>MADPSSFASPEKFNIKHMHLKLHVDFTSRAIAASTSLTVRSLQDSLASLILDTKDLTIKKVAVNGKDATFALGTTHSFKGTPLEITLPFSLTRGQEVIVEIDSVTSPKSSALQWLNKEQTAGKIHPYLFSQCQATHCRSIIPCQDTPSVKFTYYSQVSVPKELMALMSALRDGELSEQSDSNRKIYRFKQNVPIPSYLIALVVGALEGRKVGPRTTIWTEKELLEPSVYEFAETEKMLKYAEDLAGPYVWGQYDLLILPPSFPYGGMENPCLTFVTPTVLAGDRSLASVIAHEISHSWTGNLVTNETWENFWLNEGHTVYLERRIDGRLYGEEFRQFKALGGWKELQNSVNTFGATNPLTNLVPNLHEVDVDAAFSSVPYEKGFALLFYLEQLLGGPEIFLGFLKSYIQMFAFKSVTTEEWKKFLYSYFKDKVDILDKVDWKGWMHTPGMPPVQPKYDMTLANACITLGQKWVKATESDLGSFSADDVKDLSSHQLIEVLAILLLEKPLPVSHVKRMQEVYNLNDVKNSEIRFRWL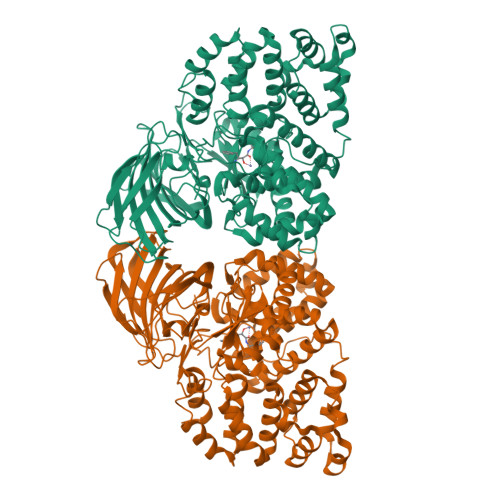RLCIRAGWEDVIPLALAMATEQGRMKFTRPLYRDLYNFEKAREQTVNTFLKNRSFMHPVTEMLVAKDLHISAS[2x]>MAKLLIMSIVSFCFIFLLLLFFRYILKRYFNYMLNYKVWYLTLLAGLIPFIPIKFSLFKFNNVNNQAPTVESKSHDLNHNINTTKPIQEFATDIHKFNWDSIDNICTVIWIVLVIILSFKFLKALLYLKYLKKQSLYLNENEKNKIDTILFNHQYKKNIVIRKAETIQSPITFWYGKYIILIPSSYFKSVIDKRLKYIILHEYAHAKNRDTLHLIIFNIFSIIMSYNPLVHIVKRKIIHDNEVEADRFVLNNINKNEFKTYAESIMDSVLNVPFFNKNIL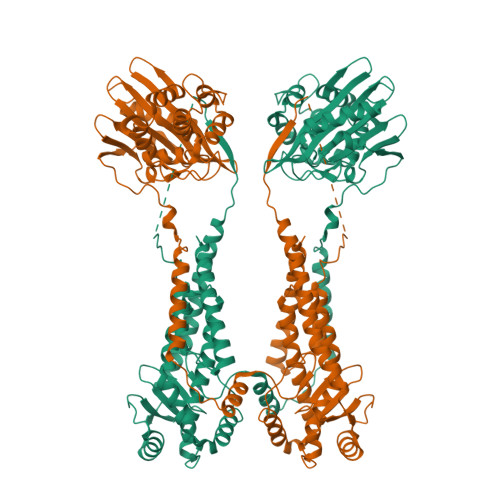SHSFNGKKSLLKRRLINIKEANLKKQSKLILIFICIFTFLLMVIQSQFLMGQSITDYNYKKPLHNDYQILDKSKIFGSNSGSFVMYSMKKDKYYIYNEKESRKRYSPNSTYKIYLAMFGLDRHIINDENSRMSWNHKHYPFDAWNKEQDLNTAMQNSVNWYFERISDQIPKNYTATQLKQLNYGNKNLGSYKSYWMEDSLKISNLEQVIVFKNMMEQNNHFSKKAKNQLSSSLLIKKNEKYELYGKTGTGIVNGKYNNGWFVGYVITNHDKYYFATHLSDGKPSGKNAELISEKILKEMGVLNGQELALVPRGSSAHHHHHH[2x]>[12x]SSTILVIHGPNLNLLGKREPEVYGHLTLDNINRQLIAQAEQASITLDTFQSNWEGAIVDRI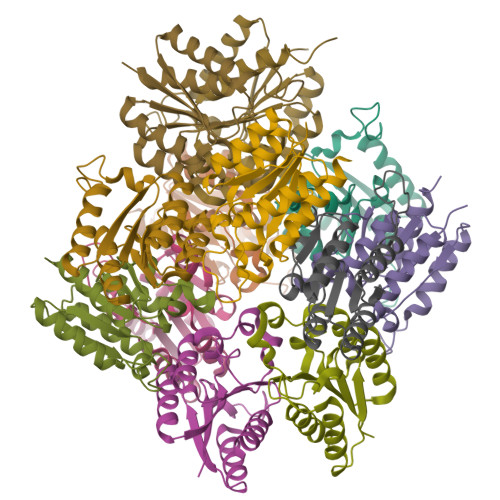HQAQTEGVKLIIINPAALTHTSVALRDALLGVAIPFIEVHLSNVHAREAFRHHSYLSDKAIGVICGLGAKGYSFALDYAIEKIQPSNPN>[4x]MKKENQTQEIEERYQALFSNAAAVKALTQVVANSLGPKGLDAMLVDRFGEVVVTNDGVTILTLMDAQHPAARMVVNMARAQEREVGDGTTTAAVLAGALVSEGVNQILKGVPVSKVLAGMNRALNHALFLIRKNAIKVGSITDDRLLAAAKIAGRGDERVAAILRDAAAMLEDKLQDPGFKLADLVLAKVGADTTLIPGVVINKSPLWEEGSQKLQEVRLLVLDDGLYPEEVEEEALASEAGFEQYLKNQKIFQENLKKLKELGVKLILLTRGISDIAEEFCYENEIMVITRITQKELKRVLEFTGARAAKRTSLNKPVEELQKMLGYARTCFYDSRLDFTIIEGGAGKATATVLIGAATDEVVDEQERIAKDAAGSFAAAYRSGVLPGGGAFFLYLSREVESLKNRLPGMESYGVMAFSEALKVPFRVMAENAGFNGLEKLGDLMTLQVQKNNYALGLDFETGEFIDMIAGGVVDPAEVVYQAVKNASEVAISLLKINTIIKMKDYEVLKEGEQEDGGKR

Here we describe the prototype crystal structures of the bacterial Group III CPN from Carboxydothermus hydrogenoformans (Ch-CPN), an extremely thermophilic, carbon monoxide utilizing bacterium isolated from a hot spring in Eastern Russia. The subunits of Ch-CPN assume the modular structure consisting of an equatorial domain, an intermediate domain, and an apical domain. Like Group II CPNs, Ch-CPN is a hexadecamer consisting of a doublet of octameric rings, its subunits interact between the rings in a direct rather than staggered subunit to subunit fashion, and achieve cavity closure independent of co-chaperones. The closed state with a non-hydrolyzable ATP analog and the open state with ADP represent the conformational states of Ch-CPN before and after ATP hydrolysis, respectively.

The crystal structure of Ch-CPN in complex with AMPPNP, an ATP analog, revealed its closed conformation. Eight subunits (from S1 to S8) assemble into a hemisphere-like complex with ~ 73 Å in height and ~ 160 Å in diameter. Two octameric hemispheres are stacked in a back-to-back manner to form a hexadecameric sphere with apical domains gathering around the two poles and equatorial domains at the equator. The stacking is mediated only by equatorial domains in such a way that each equatorial domain in one hemisphere has only one contacting partner - the S1 equatorial domain in one hemisphere directly interacts only with the S1′ equatorial domain in the opposite hemisphere. First, an inter-subunit β-sheet is constructed by the stem loop in the S1 equatorial domain and the N-/C-terminal strands in the S2 equatorial domain. AMPPNP binds to the interface between the equatorial and intermediate domains. The β- and γ-phosphates are hydrogen bonded to Asp87, Thr89, and Thr91 in a conserved P-loop motif characterized by the sequence GDGTTT29. A magnesium ion whose source seems to be the mother liquor is coordinated by the three phosphates and Asp87, which contributes to neutralization of the negative charge of phosphates. Asn55 and Asp56 in the so-called stem loop, and Arg155 and Asp373 in the intermediate domain interact with the α- and γ-phosphates of AMPPNP in C-subunit. In the closed form of Ch-CPN, eight α10 helices from each subunit are located side-by-side with no overlap at the center of the ring to close the chamber.> SGIVQQQNNLLRAIEAQQHLLQLTVWGIKQLQA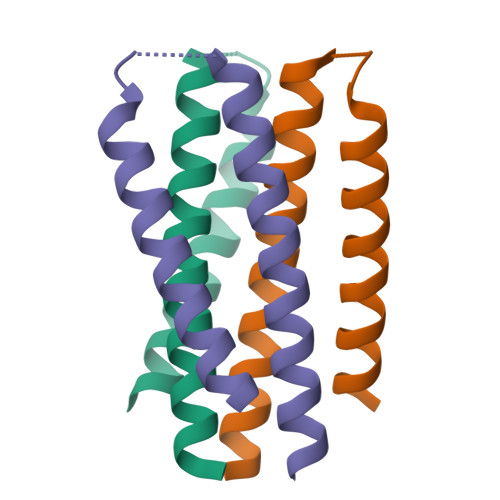RSGGRGGWMEWDREINNYTSLIHSLIEESQNQQEK>MQERILFGTYTKKTSQGIYQGTLDTTAKTLTNDGLLAATQNPTYLALSAKDCLYSVDKEDDEGGIAAWQIDGQTAHKLNTVVAPGTPPAYVAVDEARQLVYSANYHKGTAEVMKIAADGALTLTDTVQHSGHGPRPEQDGSHIHYTDLTPDNRLAVIDLGSDKVYVYNVSDAGQLSEQSVLTMEAGFGPRHLVFSPDGQYAFLAGELSSQIASLKYDTQTGAFTQLGIVKTIPADYTAHNGAAAIRLSHDGHFLYVSNRGYNTLAVFAVTADGHLTLIQQISTEGDFPRDFDLDPTEAFVVVVNQNTDNATLYARDLTS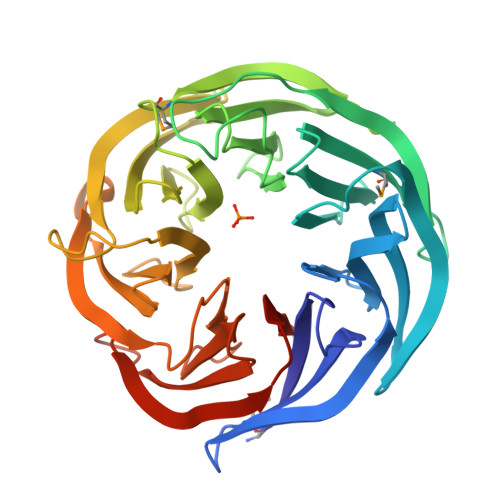GKLSLLQKDVTVPEGVCVRFLEHHHHHH[2x]>MHHHHHHENLYFQGMNDEPRWLTAEEQLVWRSYIEAATLLEDHLDRQLQRDAGMPHVYYGLLVKLAESPRRRLRMTELAKYAKITRSRLSHAVARLEKNGWVRREDCPSDKRGQFAILTDEGYEVLRRTAPGHVDAVRQAVFDR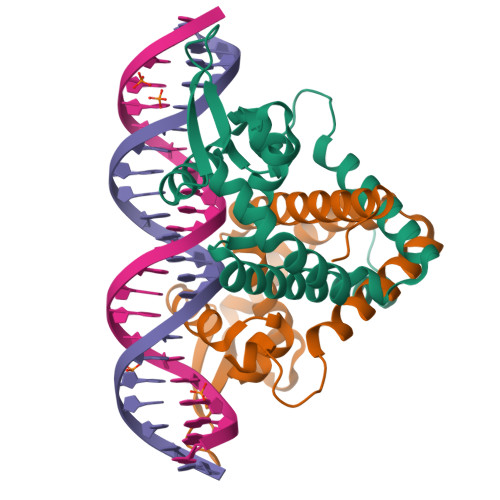LTPEQQKSLGEIMRIVAEGLQPSEAGADLPWLR[4x]>[2x]MNAAAEAEFNILLATDSYKVTHYKQYPPNTSKVYSYFECREKKTENSKVRKVKYEETVFYGLQYILNKYLKGKVVTKEKIQEAKEVYREHFQDDVFNERGWNYILEKYDGHLPIEVKAVPEGSVIPRGNVLFTVENTDPECY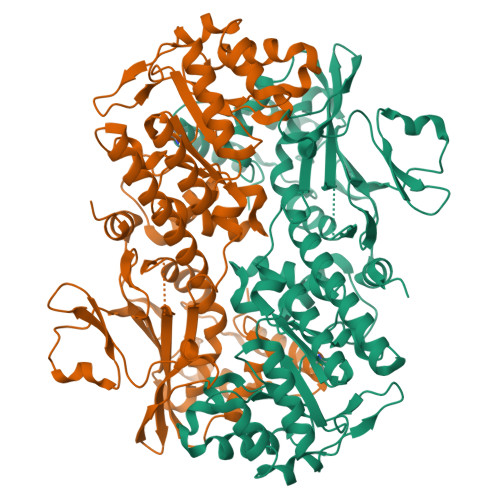WLTNWIETILVQSWYPITVATNSREQKKILAKYLLETSGNLDGLEYKLHDFGYRGVSSQETAGIGASAHLVNFKGTDTVAGIALIKKYYGTKDPVPGYSVPAAEHSTITAWGKDHEKDAFEHIVTQFSSVPVSVVSDSYDIYNACEKIWGEDLRHLIVSRSTEAPLIIRPDSGNPLDTVLKVLDILGKKFPVTENSKGYKLLPPYLRVIQGDGVDINTLQEIVEGMKQKKWSIENVSFGSGGALLQKLTRDLLNCSFKCSYVVTNGLGVNVFKDPVADPNKRSKKGRLSLHRTPAGNFVTLEEGKGDLEEYGHDLLHTVFKNGKVTKSYSFDEVRKNAQLNIEQDVAPH>MNELVDTTEMYLRTIYDLEEEGVTPLRARIAERLDQSGPTVSQTVSRMERDGLLRVAGDRHLELTEKGRALAIAVMRKHRLAERLLVDVIGLPWEEVHAEACRWEHVMSEDVERRLVKVLNNPTTSPFGNPIPGLVELGVASENLYFQGGGH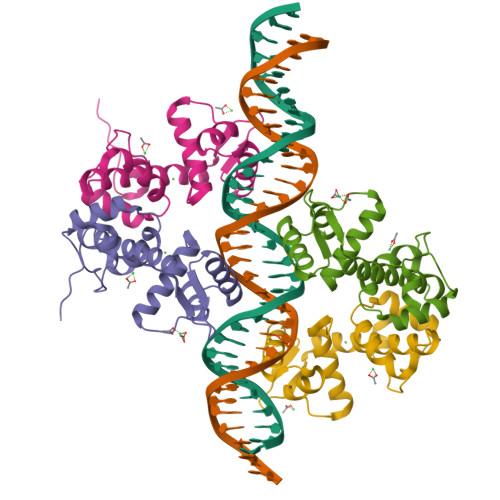HHHHH[4x]> MGALARALLLPLLAQWLLRAAPELAPAPFTLPLRVAAATNRVVAPTPGPGTPAERHADGLALALEPALASPAGAANFLAMVDNLQGDSGRGYYLEMLIGTPPQKLQILVDTGSSNFAVAGTPHSYIDTYFDTERSSTYRSKGFDVTVKYTQGSWTGFVGEDLVTIPKGFNTSFLVNIATIFESENFFLPGIKWNGILGLAYATLAKPSSSLETFFDSLVTQANIPNVFSMQMCGAGLPVAGSGTNGGSLVLGGIEPSLYKGDIWYTPIKEEWYYQIEILKLE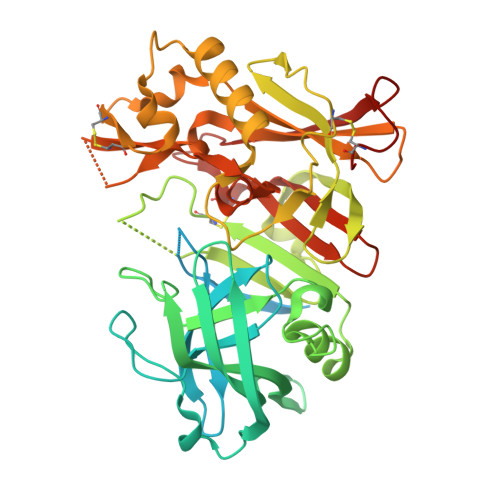IGGQSLNLDCREYNADKAIVDSGTTLLRLPQKVFDAVVEAVARASLIPAFSDGFWTGSQLACWTNSETPWSYFPKISIYLRDENSSRSFRITILPQLYIQPMMGAGLNYECYRFGISPSTNALVIGATVMEGFYVIFDRAQKRVGFAASPCAEIAGAAVSEISGPFSTEDVASNCVPA>[4x]VGAFRSGLEDKVSKQLESKGIKFEYEEWKVPYVIPASNHTYTPDFLLPNGIFVKT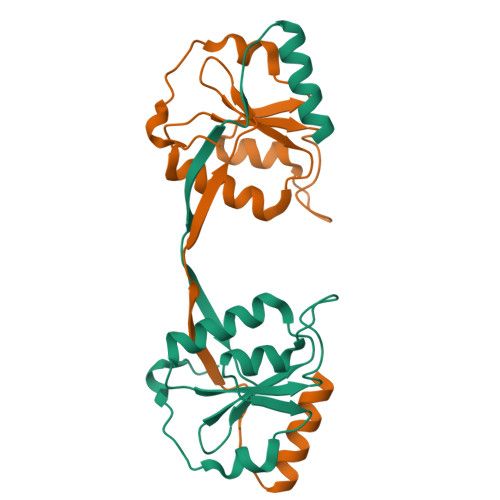KGLWESDDRKKHLLIREQHPELDIRIVFSSSRTKLYKGSPTSYGEFCEKHGIKFADKLIPAEWIKEPKKEVPFDRLKRKGGKK> SNAMYDGLSRDEQRLLNHVREYGEKYFTPASISKWRKDQGLPDEVVKAFVDLDFNGFGVIHRRNHRTYDLFAQVLVIEELSRISGACLPFQNDLLQLQ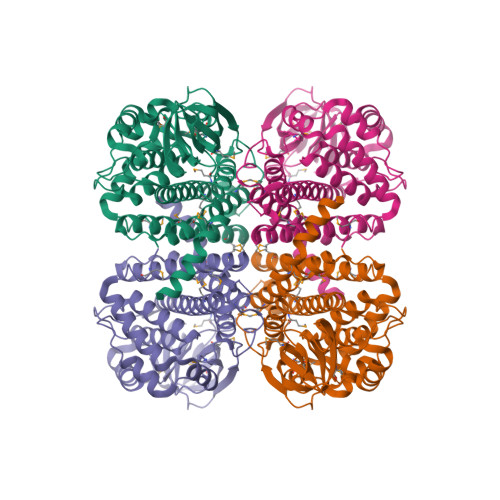ILEAFASSAQTSPFRTEYQDTGRLSYALAISEPEAGSDTRSMRTHVTREGDTLVMNGTKMFVNNGEYAPALLVSAYDKTGDDGEPEFSFWMVPRSAAGIYAYPEQKIGQSMLPFATVRFDNVEVKESWRLKGSSKGFSQLYSLLEYGRVFTCAAALGEAQAAMEDAVAWARGREAFGQRIADLQQVQMKLTEMEVKLTNMRNLVYGAAREYDRGEHKRLSVALMKYYVPKAATEVASDAMQILGGRGYIQENRVSSIWQDCRGYQFADGTDEVMVVIAAPLILEQYKASKNNR>RAGPVTWVMMIACVVVFIAMQILGDQEVMLWLAWPFDPTLKFEFWRYFTHALMHFSLMHILFNLLWWWYLGGAVEKRLGSGKLIVITLISALLSGYVQQKFSGPWFGGLSGVVYALMGYVWLRGERDPQSGIYLQRGLIIFALIWIVA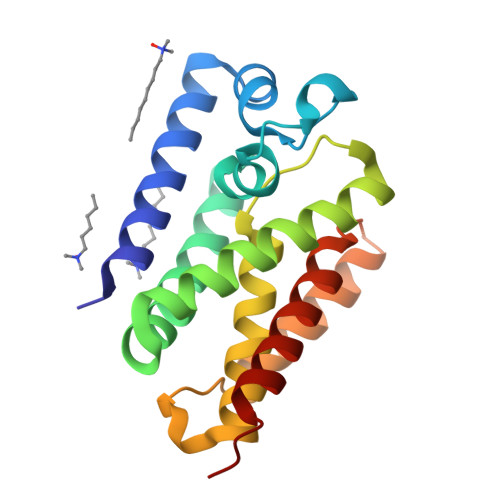GWFDLFGMSMANGAHIAGLAVGLAMAFVDSLNAR[2x]>GPGSMADPSLNNPVVIQATRLDASILPRNVFSKSYLLYVIAQGTDVGAIAGKANEAGQGAYDAQVKNDEQDVELADHEARIKQLRIDVDDHESRITANTKAITALNVRVTTAEGEIASLQTNVSALDGRVTTAENNISALQADYVSKTATTSQSLASPLNVTTSYSVGGKKVLGARQTGWTAATGTANKGVFDADLTFAVSDTYTQS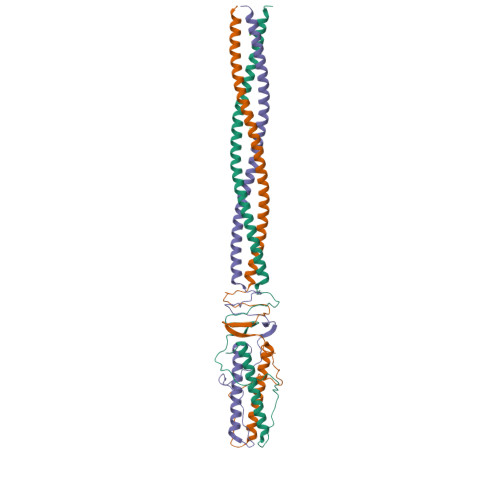EIQAIANALITERRRTKAMEDALRAHGLID[2x]> LKESPSGYLRSGEGDTGCGELVWVGEPLTLRTAETITGKYGVWMRDPKPTYPYTQETTWRIDTVG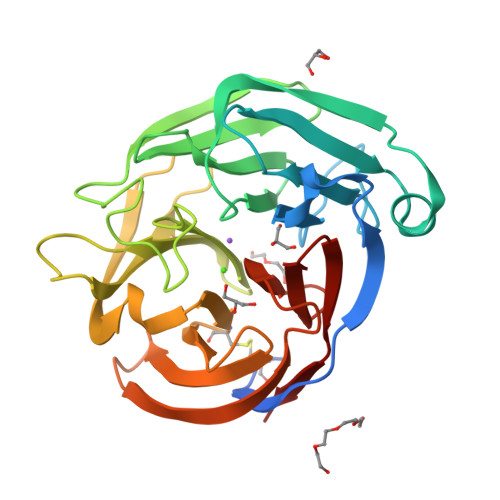TDVRQVFEYDLISQFMQGYPSKVHILPRPLESTGAVVYSGSLYFQGAESRTVIRYELNTETVKAEKEIPGAGYHGQFPYSWGGYTDIDLAVDEAGLWVIYSTDDAKGAIVLSKLNPENLELEQTWETNIRKQSVANAFIICGTLYTVSSYTSADATVNFAYDTGTGISKTLTIPFKNRYKYSSMIDYNPLEKKLFAWDNLNMVTYDIKLSKM> MILDTDYITENGKPVIR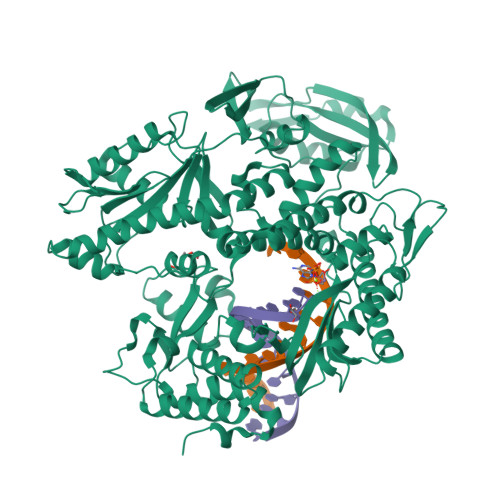VFKKENGEFKIEYDRTFEPYFYALLKDDSAIEDVKKVTAKRHGTVVKVKRAEKVQKKFLGRPIEVWKLYFNHPQDVPAIRDRIRAHPAVVDIYEYDIPFAKRYLIDKGLIPMEGDEELTMLAFAIATLYHEGEEFGTGPILMISYADGSEARVITWKKIDLPYVDVVSTEKEMIKRFLRVVREKDPDVLITYNGDNFDFAYLKKRCEELGIKFTLGRDGSEPKIQRMGDRFAVEVKGRIHFDLYPVIRRTINLPTYTLEAVYEAVFGKPKEKVYAEEIAQAWESGEGLERVARYSMEDAKVTYELGREFFPMEAQLSRLIGQSLWDVSRSSTGNLVEWFLLRKAYKRNELAPNKPDERELARRRGGYAGGYVKEPERGLWDNIVYLDFRSLYPSIIITHNVSPDTLNREGCKEYDVAPEVGHKFCKDFPGFIPSLLGDLLEERQKIKRKMKATVDPLEKKLLDYRQRAIKILANSFYGYYGYAKARWYCKECAESVTAWGREYIEMVIRELEEKFGFKVLYADTDGLHATIPGADAETVKKKAKEFLKYINPKLPGLLELEYEGFYVRGFFVTKKKYAVIDEEGKITTRGLEIVRRDWSEIAKETQARVLEAILKHGDVEEAVRIVKEVTEKLSKYEVPPEKLVIHEQITRDLRDYKATGPHVAVAKRLAARGVKIRPGTVISYIVLKGSGRIGDRAIPADEFDPTKHRYDAEYYIENQVLPAVERILKAFGYRKEDLRYQKTKQVGLGAWLKVKGKK N-(2,3-DIHYDRO-7,8-DIMETHOXYIMIDAZO[1,2-C] QUINAZOLIN-5-YL)NICOTINAMIDE 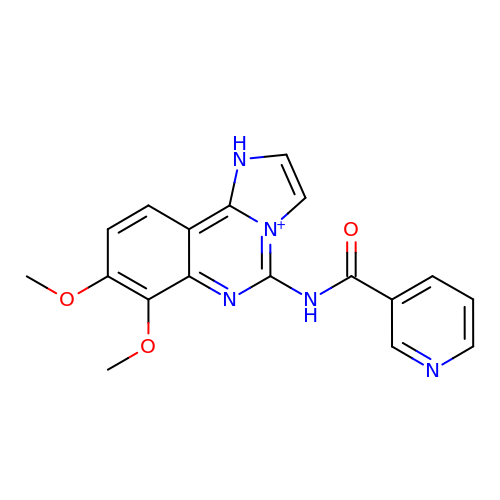| C18 H16 N5 O3 | GLZPAFCYKOIQQZ-UHFFFAOYSA-O>MFGRKKGDVIDAGAELERAEQERIEGEYGASELASERRPHTPGARTLLMVLLCVIA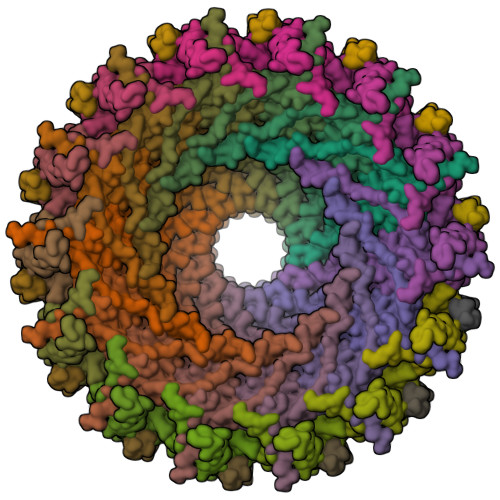VVLVTLSYKAYKVRGVVEDDDAQPQQVVRQVIPGYTPRPIRPEPENVPEPPQPTTSVPAIQPAPVTQPVRPQPTGPREKTPYELARERMLRSGLTAGSGGGEDLPRPQGGDVPAGGLMGGGGGGGELAEKLQPMRLSGSSAGRLGNRDMLITQGTQLDCVLETRLVTTQPGMTTCHLTRDVYSTSGRVVLLDRGSKVVGFYQGGLRQGQARIFVQWSRIETPSGVVINLDSPGTGPLGEAGLGGWIDRHFWERFGGAIMISLIGDLGDWASRQGSRQGDNSIQFSNTANGVESAAAEALRNSINIPPTLYKNQGERVNILVARDLDFSDVYSLESIPTK[14x];>[14x]MKKLAIVALLASLHAVPALALDVPSSSRYDHRIRYVTYNPADVVQVDTVLGVATHIMLEEGEQYLTHAFGDSEAYAFARKGRHIFIKPQAELANTNLIVVTDRRSYKFRLQMRNDRNGAMYELAFRYPDTQARQTREANARAAVEAAFEQRVGAYYNLKYMMSGDKDIAPVNAWDDGRFTYFKFSANADLPSIYFVDAEGNESLVPRTTVGSSNNIIAVHKVNPKWMIRLGNRALAIFNEAYDPNGVPNDTGTASPAVRRVNKGGN;>MKTIIFAILMTGLLSACASAPKPKQPSDFNREPVNKTVPVEIQRGAL[14x]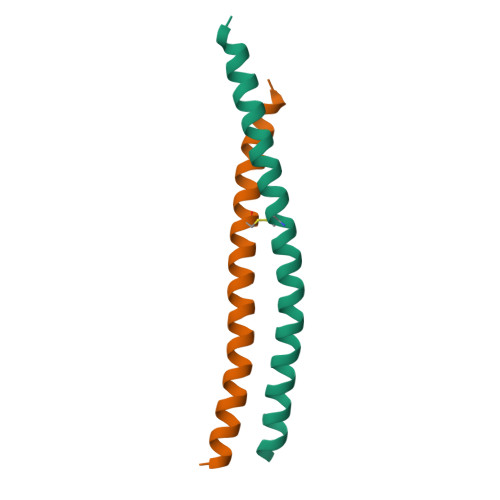>[2x]GSNNELYLELMKLREHSDQHVKELKTSLKKCARETADLKFLNNQYAHKLKLLEKESKAKNERIQQ> MITTPLVHVASVEKGRSYEDFQKVYNAIALKLREDDEYDNYIG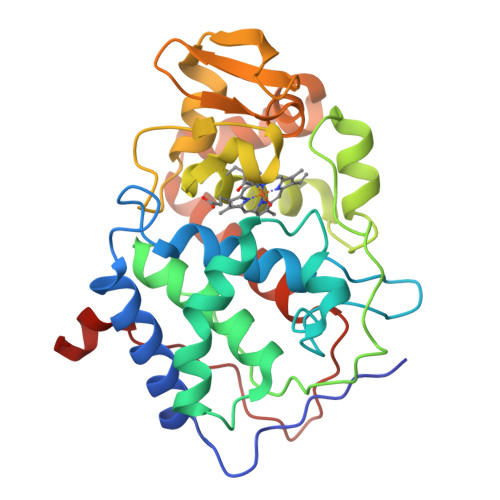YGPVLVRLAWHISGTWDKHDNTGGSYGGTYRFKKEFNDPSNAGLQNGFKFLEPIHKEFPWISSGDLFSLGGVTAVQEMQGPKIPWRCGRVDTPEDTTPDNGRLPDADKDAGYVRTFFQRLNMNDREVVALMGAHALGKTHLKNSGYEGPGGAANNVFTNEFYLNLLNEDWKLEKNDANNEQWDSKSGYMMLPTDYSLIQDPKYLSIVKEYANDQDKFFKDFSKAFEKLLENGITFPKDAPSPFIFKTLEEQGL In the periplasm, M is randomly epimerized to G or partially acetylated, and the mature alginate is directed to the transmembrane β-barrel protein AlgE in the outer membrane for conveyance to the extracellular space. Briefly, the structures include 18 antiparallel strands (S1–S18) that cross the membrane to varying degrees, nine extracellular loops (L1–L9) and eight periplasmic turns (T1–T8). The loops and turns range in size from two to 43 residues, with L1 coordinating a calcium ion. Both the N- and C-termini are in the periplasm. The cavity within the AlgE barrel has been proposed to act as a pore for alginate, a random, linear copolymer of 1,4-linked β-d-mannuronic acid (M) and its C-5 epimer α-l-guluronic acid (G).

The best crystals were obtained with 7.8 MAG at 20°C. These yielded three crystal forms in space groups C2, P212121, P21 that diffracted to 1.9, 2.4 and 2.8 Å resolution, respectively. In contrast, the asymmetric units of AlgE-2.4 and AlgE-2.8 contain two molecules (molecules A and B). For all in meso structures, type I packing was observed, as is the norm for crystals grown in a lipidic mesophase environment. Interestingly, we find that L2 and T8, while ordered in some crystal forms, are disordered in others. Disorder, where electron density is either not observed or is ill-defined in the map, suggests that the corresponding loops, or parts thereof, are flexible and, in certain cases, may have relocated to reside outside the barrel. It appears therefore that in this collection of six models we have an ensemble of structures that map a conformational landscape for alginate transport. We refer to this as the double-gate model.

>[2x]ANSGEAPKNFGLDVKITGESENDRDLGTAPGGTLNDIGIDLRPWAFGQWGDWSAYFMGQAVAATDTIETDTLQSDTDDGNNSRNDGREPDKSYLAAREFWVDYAGLTAYPGEHLRFGRQRLREDSGQWQDTNIEALNWSFETTLLNAHAGVAQRFSEYRTDLDELAPEDKDRTHVFGDISTQWAPHHRIGVRIHHADDSGHLRRPGEEVDNLDKTYTGQLTWLGIEATGDAYNYRSSMPLNYWASATWLTGDRDNLTTTTVDDRRIATGKQSGDVNAFGVDLGLRWNIDEQWKAGVGYARGSGGGKDGEEQFQQTGLESNRSNFTGTRSRVHRFGEAFRGELSNLQAATLFGSWQLREDYDASLVYHKFWRVDDDSDIGTSGINAALQPGEKDIGQELDLVVTKYFKQGLLPASMSQYVDEPSALIRFRGGLFKPGDAYGPGTDSTMHRAFVDFIWRF>MQGDPEVIEFLNEQLTAELTAINQYFLHAKLQDHKGWTKLAKYTRAESFDEMRHAEVLTDRILLLDGLPNYQRLFHVRVGQSVTEMFQADREVE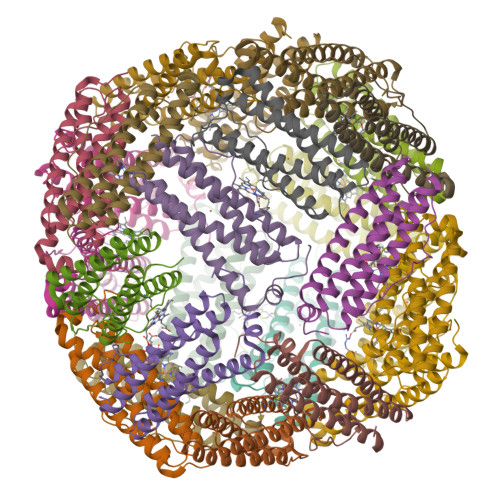LEAIDRLRRGIEVMRAKHDITSANVFEAILADEEHHIDYLETQLDLIEKLGESLYLSTVIEQTQPDPSGPGSL[24x]4-{[(3R)-4-cyclopentyl-1,3-dimethyl-2-oxo-1,2,3,4-tetrahydropyrido[2,3-b]pyrazin-6-yl]amino}-N-(1-methylpiperidin-4-yl)-3-[(propan-2-yl)oxy]benzamide | C30 H42 N6 O3 | 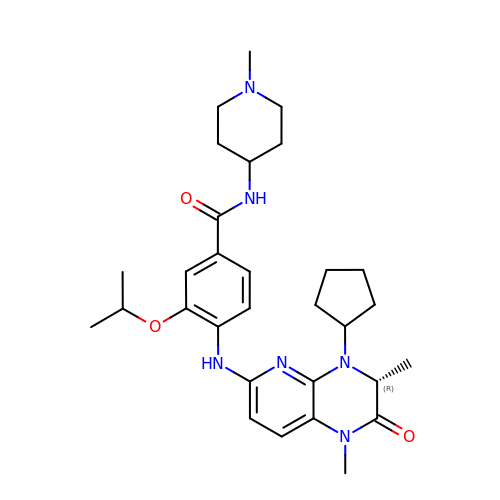AGCMTUNUCHFYSQ-HXUWFJFHSA-N The TRAPP complexes are nucleotide exchange factors that play essential roles in membrane traffic and autophagy. TRAPPII activates Rab11, and TRAPPIII activates Rab1, with the two complexes sharing a core of small subunits that affect nucleotide exchange but being distinguished by specific large subunits that are essential for activity in vivo. We report a cryo‐EM structure of the entire Drosophila TRAPPIII complex. The TRAPPIII‐specific subunits TRAPPC8 and TRAPPC11 hold the catalytic core like a pair of tongs, with TRAPPC12 and TRAPPC13 positioned at the joint between them.

However, in the regions of TRAPPC8 and TRAPPC11 located on either side of the core the local resolution was suitable for de novo model building. An α‐solenoid is also seen for TRAPPC11, with residues 181–566 forming fifteen α‐helices that includes the interaction surface with TRAPPC2L. This region of TRAPPC11 has been referred to as the “foie gras domain” after the zebrafish gene in which it was first analysed as it was noted to be particularly well conserved between species (Pfam domain PF11817). The N‐terminal part of TRAPPC11 (residues 1–180) consists of four β‐strands interspersed with four α‐helices. The C‐terminal part (residues 567–1,320) is less well resolved but forms the arm connecting to the vertex with TRAPPC12 and TRAPPC13. The surface of interaction between TRAPPC2L and TRAPPC11 has a total area of 558 Å. The overall arrangement of the interaction is similar to that of TRAPPC2 and TRAPPC8 (Fig EV2A). As was seen with TRAPPC2, α‐helix 1 of TRAPPC2L is central to the interface and interacts with α‐helices 14 and 15 of the TRAPPC11 α‐solenoid. We could identify two conserved regions in TRAPPC11 that are involved in the interaction. α‐helix 14 (Tyr442 to Ile453) contacts TRAPPC2L between Asn33 and Lys42. The other region is between residues Asp478 to Thr486 at the end of α‐helix 15, where residues such as Trp484 contact TRAPPC2L α‐helix 1 and the loop between β‐strands 1 and 2, similar to TRAPPC8 and TRAPPC2.

> MTMDATALPSELLVTPQPLVGFCGLDTARVSVHKAVWEAFSGSLQRKAADRAAVQYKLLPPNYEFPVAKPKRASYEWYHPKGILKRNWMLKHLHVLPSVVVLFQDMEWNDLQWTEKQVQCAAIVQALKNTLQERNTRLCLVLLQRAAPLPPGEDLLAAERAASLTNACGITSKMLFILPHTEHLTGYALRLESAFLDMAQSYYALMSKRIRNHRDQLTAAHTSLKIRHQFKLGFVAEMRQDFSTGQKHYFQAYANLDEIRINDGNCLEIKTLAGFLNYKICRLMFKLKTPRDAINQFIIHVEKHKSRVGFKDLAFEHHAWLSTQHSVFAELFCEAIKNGLPALQTQHPGIYYHKAAEFVMKRRDAAMEAYAAMQASSEATPTPIQNPLSLYTEFFGIRAVKTGDLVAEQQANMQLCDQERSYNHSAAIIALLSQAMAQFKIYKCLRFRKKLAIDMAEEYLKSGDHAKALTLYSLMLPDYRQEKWTTIFTDVLLKTLRCALLSGSVADYIACSVEALSLRHQSDQSERILILENLWQVFQGVPPMPKTQLTPEAQALWTSALANVKSPIQIDLDKVNDVVEMCATFERVQLSNDDLLQLQLIVRVLTDIPLRIRSFHVILADAGNPQNSYKLEALKYFCFPTLTQLRGQKQPDDEQLENPSQEPKNFEKNMRLEPGSYYQLFCSTEAQQFHENTQLRIVRLEAHMGTDQVAALLTCSSN N-ethyl-2-(1-methyl-1H-1,2,3-triazol-4-yl)-6-(1-phenylethyl)isonicotinamide 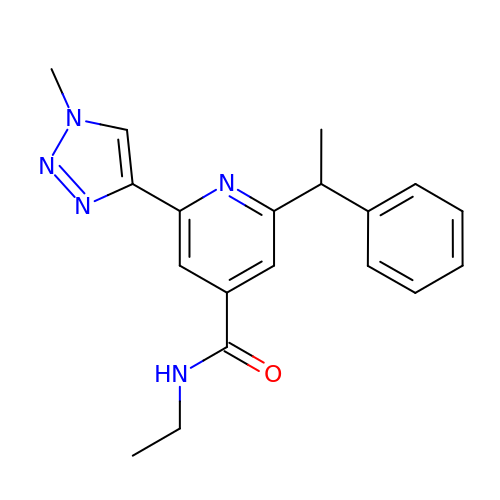| C19 H21 N5 O | LOEKXZDIARTPMM-ZDUSSCGKSA-N4-methyl-6-{[3-(piperidin-4-ylmethoxy)phenoxy]methyl}pyridin-2-amine 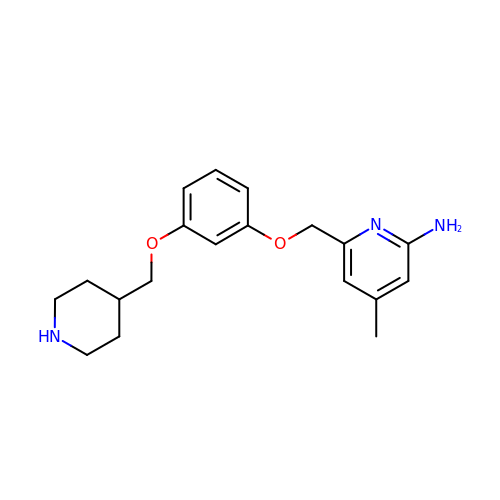| C19 H25 N3 O2 | PXVODVINMZHSGT-UHFFFAOYSA-N>MNRQIVRSALFVPATRPERIPKALASGADRVIVDLEDAVEEGLKVEARANLRRFLVDTPEARVLVRINAAEHPG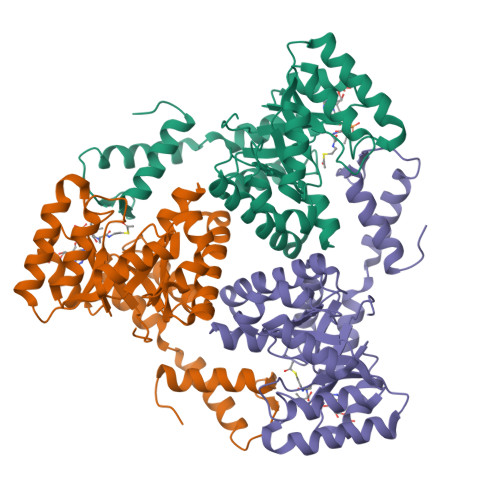HADDLALCRDHAGVIGLLLPKVESAAQVRHAAVASGKPVWPIVESARGLAALGEIAAAAGVERLSFGSLDLALDLDLNSGSNAAEQILGHARYALLLQTRLAGLAPPLDGVYPAIQNRAGLVEAVRFARDMGFGGLLCIHPSQVEPIHQTLMPSPAELEWARRVAEAGASGAGVFVVDGEMVDAPVLGRARRLLERAGEGG[3x]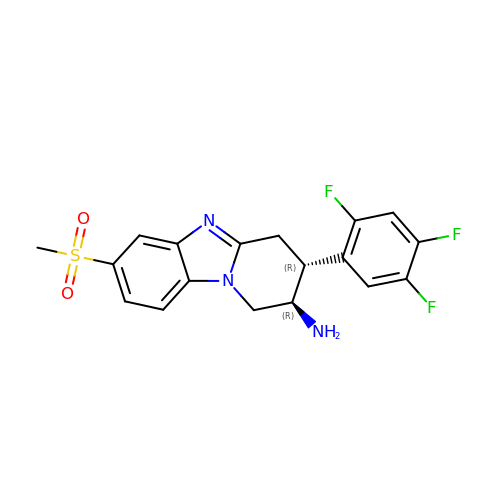(2R,3R)-7-(methylsulfonyl)-3-(2,4,5-trifluorophenyl)-1,2,3,4-tetrahydropyrido[1,2-a]benzimidazol-2-amine | C18 H16 F3 N3 O2 S | HJJAYSSCWGUPKO-ABAIWWIYSA-N FN558 | C24 H21 F6 N O2 | 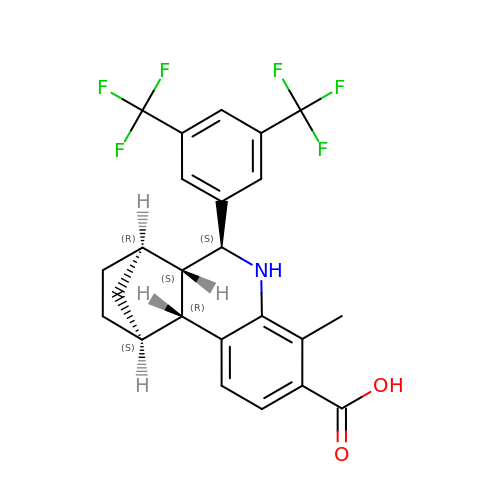ZDLBBVTYBSLWNB-PSPNCCEFSA-N>[2x]TRDQNGTWEMESNENFEGYMKALDIDFATRKIAVRLTQTKVIDQDGDNFKTKTTSTFRNYDVDFTVGVEFDEYTKSLDNRHVKALVTWEGDVLVCVQKGEKENRGWKQWIEGD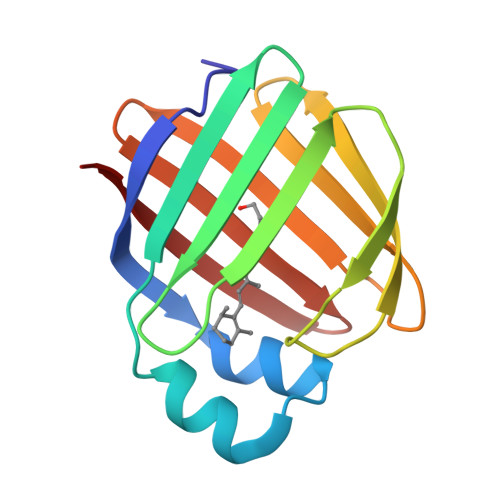KLYLELTCGDQVCRQVFKKK> MASVDFKTYVDQACRAAEEFVNVYYTTMDKRRRLLSRLYMGTATLVWNGNAVSGQESLSEFFEMLPSSEFQISVVDCQPVHDEATPSQTTVLVVICGSVKFEGNKQRDFNQNFILTAQASPSNTVWKIASDCFRFQDWAS;> APPCKGSYFGTENLKSLVLHFLQ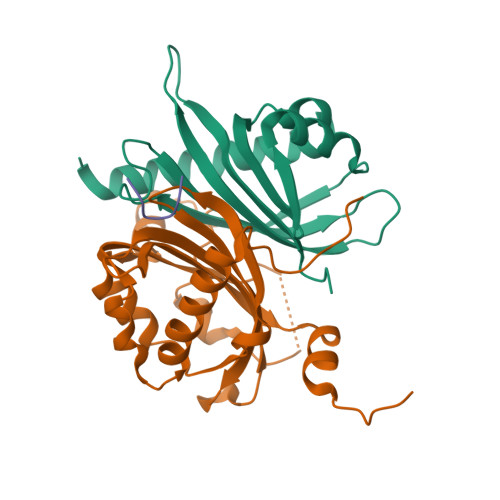QYYAIYDSGDRQGLLDAYHDGACCSLSIPFIPQNPARSSLAEYFKDSRNVKKLKDPTLRFRLLKHTRLNVVAFLNELPKTQHDVNSFVVDISAQTSTLLCFSVNGVFKEVDGKSRDSLRAFTRTFIAVPASNSGLCIVNDELFVRNASSEEIQRAFAMPAPTPSSSPVPTLSPEQQEMLQAFSTQSGMNLEWSQKCLQDNNWDYTRSAQAFTHLKAKGEIPEVAFMK;> GQSPGFGQGGSV>SLINTKIKPFKNQAFKNGEFIEVTEKDTEGRWSVFFFYPADFTFVCPTELGDVADHYEELQKLGVDVYSVSTDTHFTHKAWHSSSETIAKIKYAMIGDPTGALTRNFDNMREDEGLADRATFVVDPQGII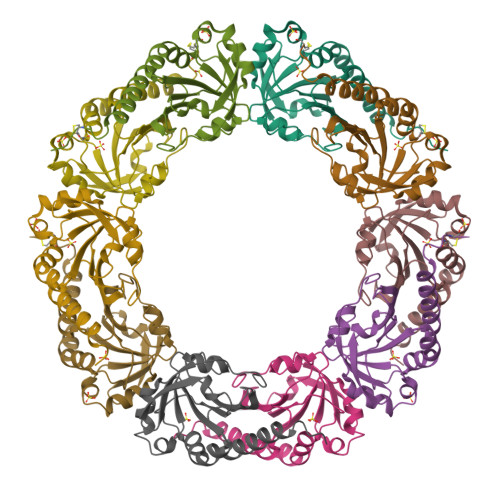QAIEVTAEGIGRDASDLLRKIKAAQYVAAHPGEVCPAKWKEGEATLAPSLDLVGKI[5x]> GAMGDEVVVDHAATKR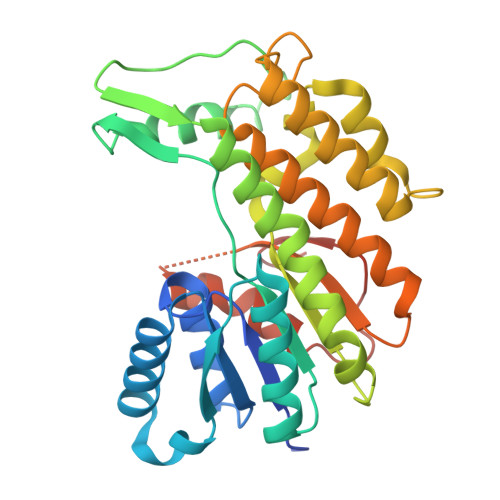YAVVTGANKGIGFEICKQLASKGITVILASRDEKRGIEARERLIKELGSEFGDYVVSQQLDVADPASVAALVDFIKTKFGSLDILVNNAGLNGTYMEGDASVLNDYVEAEFKTFQSGAAKTEPYHPKATGRLVETVEHAKECIETNYYGSKRVTEALIPLLQQSDSPRIVNVSSTLSSLVFQTNEWAKGVFSSEEGLTEEKLEEVLAEFLKDFIDGKQQEKQWPPHFSAYKVSKAALNAYTRIIAKKYPSFRINAVCPGYTKTDLSYGHGQFTDAEAAEAPVKLALLPQGGPSGCFFFRDEAFCLYLE>[2x]SNADRWPLSYAQQRLWFLAQMGQAASSAYHIAGGLTLRGHLDEGALQAALDRIVQRHEALRTRFELQDGQPVQRIDAPRPFALFRQALGAGEAELAHWQQVEAQTPFDLGTGPLIRGRLLKRNEQEHVLLLTMHHIVSDGWSMGVLARELGALYRAYAEEKIGPEIDPLPALPLQYADYA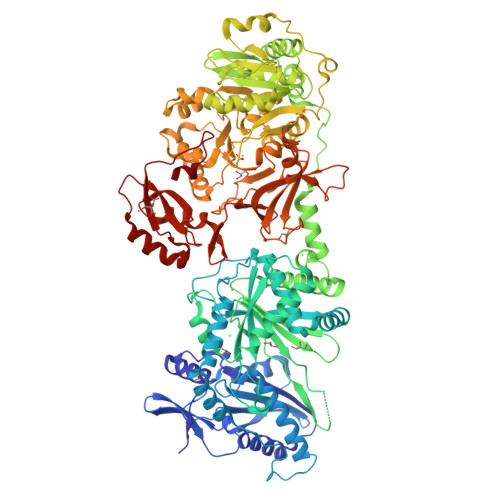VWQRRWLNGELQQRQLAYWQQQMAGAPALVSLPTDRPRPALQDYRGEVVDIELDAALSAGLKRLSQRHGTTLYMTVLAAWAALVARLAGQSEVVIGSPVANRQRAELEGLIGFFVNTLALRIDLGGDPSVAQLLAQVRERVLAAQSHQDLPFEQVVEALKPERSLSHSPVFQLMLSWQSGPQPGLKLGGLGLDALPAGSRRSAQFDLSLELQDRGDGTIAGSLTYASALYERETVQRHAGYLKALLAGMAADDTQPVQRIGILGEAERHRLLVEWNDTAREHPRTVCVHELFEQQVERSPEAVALVYEGQQLSYRELDRQANRLARQLKALGVGPDERVAVCTERCLEMVVALLAVLKAGGAYVPLDPGYPAERLEYMLADSAPKVLLRQSGQTLEPGAGVAVLALDGEASQPWQAQPAQRLSRDDSGVQPHHLAYVIYTSGSTGRPKGVMVEHAGVVNRLLWMQRAYGLQPQEAVLQKTPFGFDVSVWEFFWPLAVGARLVMARPQGQQDPAYLVETIVGQDIGTLHFVPSMLQAFVDSEGVQRCRGVRRIVCSGEALPGALARRLRQQLPQVELHNLYGPTEATVDVTAWACDAAELPDNIPIGRPVDNTTMYVLDAHGQPVPTGVAGEIHIGGVQVARGYLGRPELTRERFVPDPYAGRPGARLYKTGDLGRWLPDGTLEYLGRNDHQVKIRGLRIELGEIEAQLARQPGVREAVVLARQDRPGDPRLVAYLLAEPAAAPDAQVLRAALMQVLPEYMVPAAYVAMPAWPLTPNGKLDRKAL>[2x]ARPCIPKSFGYSSVVCVCNATYCDSFDPPTFPALGTFSRYESTRSGRRMELSMGPIQANHTGTGLLLTLQPEQKFQKVKGFGGAMTDAAALNILALSPPAQNLLLKSYFSEEGIGYNIIRVPMASCDF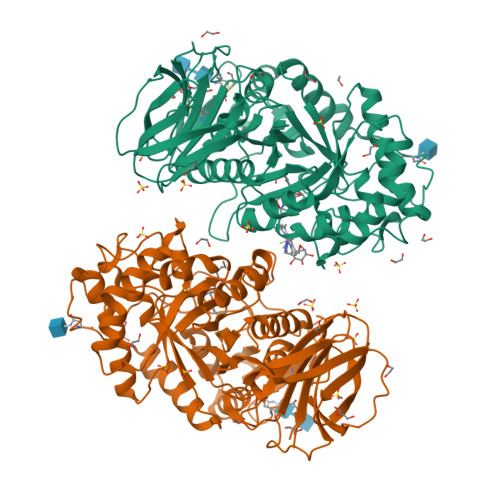SIRTYTYADTPDDFQLHNFSLPEEDTKLKIPLIHRALQLAQRPVSLLASPWTSPTWLKTNGAVNGKGSLKGQPGDIYHQTWARYFVKFLDAYAEHKLQFWAVTAENEPSAGLLSGYPFQCLGFTPEHQRDFIARDLGPTLANSTHHNVRLLMLDDQRLLLPHWAKVVLTDPEAAKYVHGIAVHWYLDFLAPAKATLGETHRLFPNTMLFASEACVGSKFWEQSVRLGSWDRGMQYSHSIITNLLYHVVGWTDWNLALNPEGGPNWVRNFVDSPIIVDITKDTFYKQPMFYHLGHFSKFIPEGSQRVGLVASQKNDLDAVALMHPDGSAVVVVLNRSSKDVPLTIKDPAVGFLETISPGYSIHTYLWHRQ> ITGQAACPE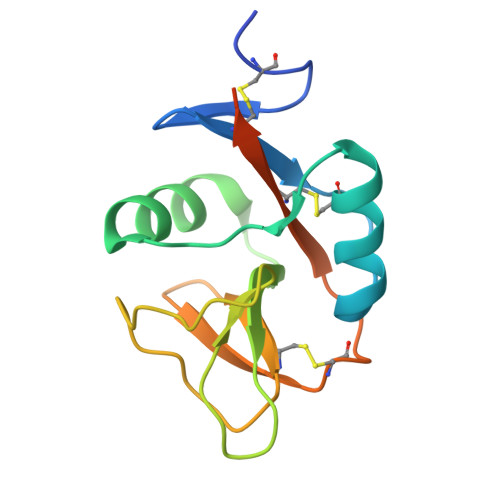SWIGFQRKCFYFSDDTKNWTSSQRFCDSQDADLAQVESFQELNFLLRYKGPSDHWIGLSREQGQPWKWINGTEWTRQFPILGAGECAYLNDKGASSARCYTERKWICSKSDIHVGTKHHHHHHHHG>MEYIIKNGFVYCPLNGVDGEKMDICVKDGKIVESVSDSAKVIDASGKIVMPGGVDPHSHIAGAKVNVGRMYRPEDSKRDAEKFKGGRAGSGFSVPSTFMTGYRYAQMGYTTAMEAAMPPLLARHTHEEFHDTPIIDHAAYPLFGNNWFVMEYLKEGDVDACAAYASWLLRATKGYTIKIVNPAGTEAWGWGGNVHGIYDPAPYFDITPAEIIKGLAEVNEKLQLPHSIHLHCNDLGHPGNYETTLASFDVPKNIKPNPATGSRDTVLYATHVQFHSYGGTTWRDFVSEAPKIADYVNKNDHIVIDVGQITLDETTTMTADGPMEYDLHSLNGLKWANCDVELETGSGVVPFIYSARAPVPAVQWAIGMELFLLIDNPEKVCLTTDSPNAGPFTRYPRVIAWLMSNKYRMNLIEGELHKWAQRKSTVATIDREYTFSEIAQITRATSAKVLGLSDTKGHLGVGADADIAVYDINPETVDPSAEYMAIEEAFSRAACVLKDGEIVVKDGEVVASPHGRTYWVDTQVDESIYSEVLANVESKFKQYYSVNFANYPVQDDYLPKSAPVKGVML[8x];>[8x]MEYVKNVVCPFCGTLCDDIICKVEGNEIVGTINACRIGHSKFVHAEGAMRYKKPLIRKNGEFVEVSYDEAIDKAAKILAESKRPLMYGWSCTECEAQAVGVELAEEAGAVIDNTASVCHGPSVLALQDVGYPICTFGEVKNRADVVVYWGCNPMHAHPRHMSRNVFARGFFRERGRSDRTLIVVDPRKTDSAKLADIHLQLDFDRDYELLDAMRACLLGHEILYDEVAGVPREQIEEAVEVLKNAQFGILFFGMGITHSRGKHRNIDTAIMMVQDLNDYAKWTLIPMRGHYNVTGFNQVCTWESGYPYCVDFSGGEPRYNPGETGANDLLQNREADAMMVIASDPGAHFPQRALERMAEIPVIAIEPHRTPTTEMADIIIPPAIVGMEAEGTAYRMEGVPIRMKKVVDSDLLSDREILERLLEKVREYKASK;>[8x]MSEIILTPKEQPEVPLEAPNIKPDVFAGKSIEEIKNIQIMHGNEVVKLGDFFEVSGEPADAPEDIKIIIDGDVYNTKRIGQEMTAGEIIVRGNVNMYVGAGMKGGKITVEGNAGSWAGQDMRGGEIEILGDAGDYVG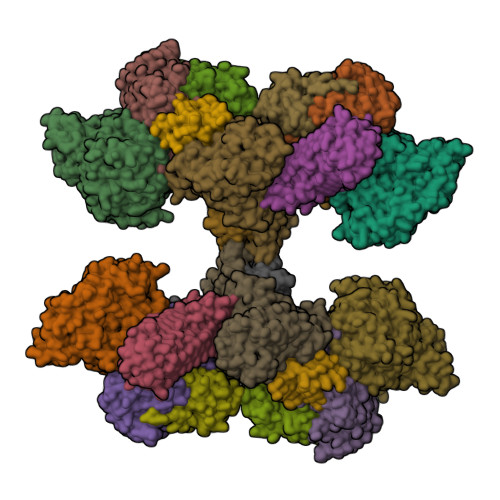SSYRGDWRGMSGGTITVHGNADNEIGEYMNGGKIIIKGDVNIMPGIHMNNGLIIIEGNVVARAGGEMAGGTIVVKGMMQEFLAGFKYLGVEKDIEVDGEELPGAFYKFEGDHAIKGAKGIVYAAVGCNGHIAP;>MRVILNTGRTIWQGQAIESGKDLKMYVDAAAIIQMNPEMMKQLGIAEGDNVKVISEYGDVVVKAVEAKEPLPEGMVYIPMGPWANRVIRPYTDSTATPSFKNIPVEIIPTDEEVLDMPTLMKVYGKVGQI[8x];>[8x]MAIGLKAYPELCHGCGNCVIACPVNALRSPEVAGGKGPTDDVEIIMIVEDGVVNIKNPDLCGKCGTCVESCPVDAIRLEELE;>[8x]METTEVIEGKNITVERTGEENRRLIFQDCLCAVCGLCGEICPVSAIEVNPTGAMVRTEQEKSKIAIDENKCVLCGMCSSICPFQALDLQIDGTSIKELAEYPKIIKSAEIDDETCIQCKACETACPQDAITITRELPERKDLVTGEIEIDKDTCIYCGMCEEMCPVDAIEIDHQTPSSASPVVATDIRVDEDKCVHCGICKRICPVDAIMQVCRICPYGEYEIKTPEVTGTSYIDPELCVNCGWCQEICPVDAATVTKPFEGELIIDQDTCQACETCVMVCPCNVLSFPKPEKPGEKTTKLHKDERFCIYCGACERSCPVTAITVKRNRINTTPIRSKAWKNAFDSLLK>[4x]MIIGYARVSSLDQNLERQLENLKTFGAEKIFTEKQSGKSIENRPILQKALNFVEMGDRFIVESIDRLGRNYNEVIHTVNYLKDKEVQLMITSLPMMNEVTGNPLLDKFM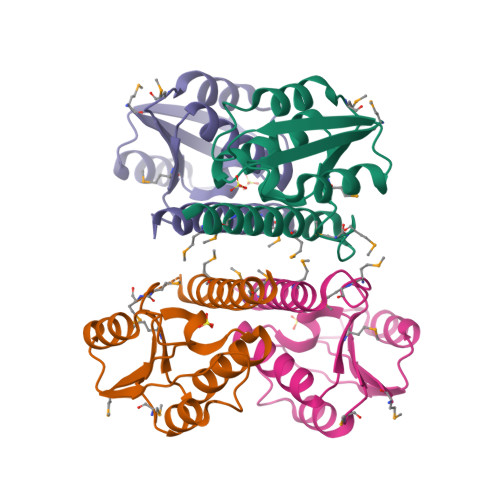KDLIIQILAMVSEQERNES> SMEPKIK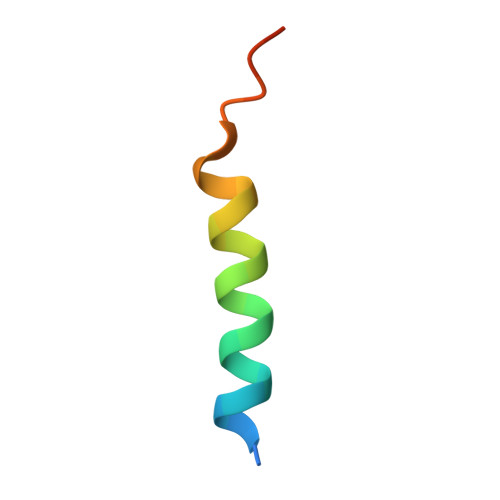EDADNAMLDSLLADPFENNSP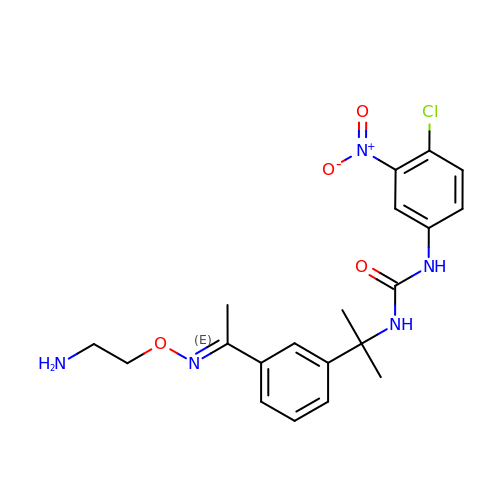1-(2-{3-[(1E)-N-(2-aminoethoxy)ethanimidoyl]phenyl}propan-2-yl)-3-(4-chloro-3-nitrophenyl)urea | C20 H24 Cl N5 O4 | MAIRRISEQUGPIE-DHRITJCHSA-N> ETMTEEQSQSFLTEFINYIKQSKVVLLEDLASQVGLRTQDTINRIQDLLAEGTITGVIDD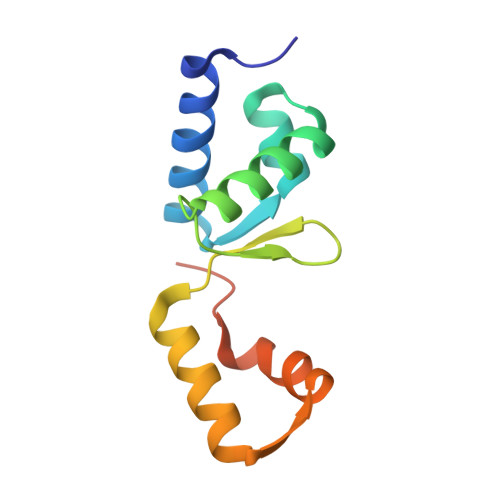RGKFIYITPEELAAVANFIRQRGRVSIAELAQASNSLIAWGRESPAQAPA>[2x]GPGYQMDIPKFKRLPRHIAIIPDGNRRWALARGLEKHEGYSSGIIPGLEVYD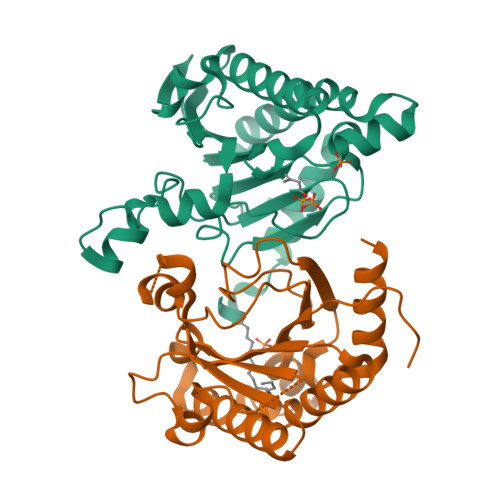ICVKIGIGEVTFFGFTQDNTKRPQIQRKAFTDACIKSVQEIAKRDAEILVVGNTNSDIFPEELLEYTKRTKVGKGKIKINFLINYGWYWDLTYAYDNSPDGKKMIENIASAEIPRVDLLIRWGGRCRLSGMLPVQTVYSDIYVVDEMWPDFKPEHLFKALEFYQNQDITLGG> MEGGGKPNSSSNSRDDGNSVFPAKASATGAGPAAAEKRLGTPPGGGGAGAKEHGNSVCFKVDGGGGGGGGGGGGEEPAGGFEDAEGPRRQYGFMQRQFTSMLQPGVNKFSLRMFGSQKAVEKEQERVKTAGFWIIHPYSDFRFYWDLIMLIMMVGNLVIIPVGITFFTEQTTTPWIIFNVASDTVFLLDLIMNFRTGTVNEDSSEIILDPKVIKMNYLKSWFVVDFISSIPVDYIFLIVEKGMDSEVYKTARALRIVRFTKILSLLRLLRLSRLIRYIHQWEEIFHMTYDLASAVVRIFNLIGMMLLLCHWDGCLQFLVPLLQDFPPDCWVSLNEMVNDSWGKQYSYALFKAMSHMLCIGYGAQAPVSMSDLWITMLSMIVGATCYAMFVGHATALIQSLDSSRRQYQEKYKQVEQYMSFHKLPADMRQKIHDYYEHRYQGKIFDEENILNELNDPLREEIVNFNCRKLVATMPLFANADPNFVTAMLSKLRFEVFQPGDYIIREGAVGKKMYFIQHGVAGVITKSSKEMKLTDGSYFGEICLLTKGRRTASVRADTYCRLYSLSVDNFNEVLEEYPMMRRAFETVAIDRLDRIGKKNSILLQKFQKDLNTGVFNNQENEILKQIVKHDREMV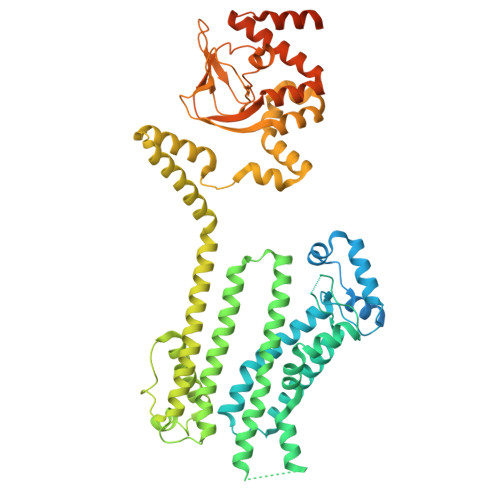QAALPRESSSVLNTDPDAEKPRFASNL>DRHHHHHHKLKDIRHSSDDDLLLPYTKSHGPSHSHRY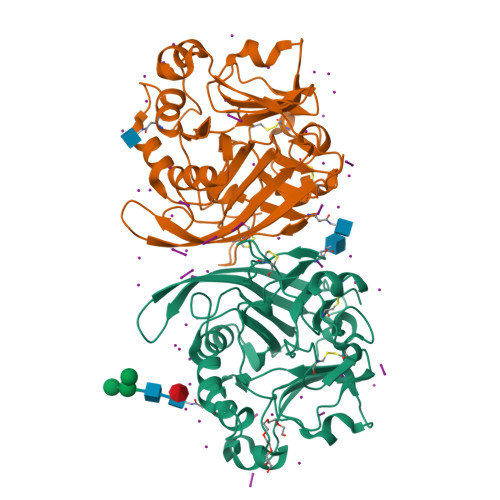VRDCQPVAHGTVTHETQAASKHSNSPVLESNIFISDITDDSGTHRWVSGHITEVHDPLRSVSVLEPGGPGGCAHNHRELVEVTAKTRKCLVAQNGGYFDTHTGQCLGNIISDGKLVRNSGGIQNAQFGIRKDGTLVFGYLSEDDILDQENPFVQLISGVVWLLRKGEIYINESIQAECDKTQETGNFRHFVDVISARTAVGHDKEGKLILFHVDGQTDVRGMNLWQVAKFLKDQNVMNAINLDGGGSATYVLNGSLASYPSDHCNPSKWRCPRAISTVLCIHER[2x]> MDTNQKLSIAVFALGCFWGPDAQFGSIKGVVSTRVGYAGGTTNNPSYYNLGDHSESIEIQYDANVITYGELLNIFWNLHNPVYETTNRQYMSRIFYLDDGQKSEALEMKRQIEAANGEKIYTEIVPLENFYLAEGYHQKYYLQNTTKLYQTLKAIYGGFGNLVRSTLAARMNGYIAGNLSIASLKEEMDLVELPEDQYEKVLSIVEEI;>MAKEVIVYTSNTCPHSFTVKEF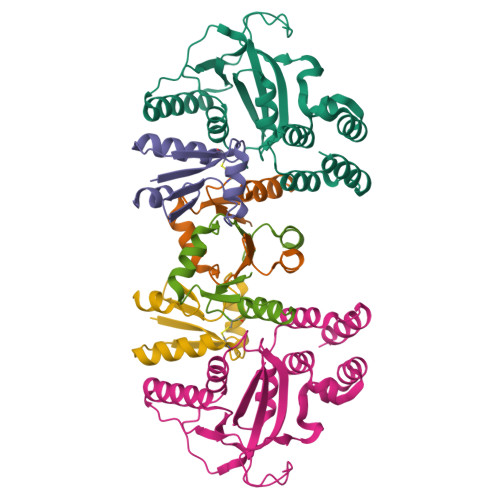LSENNVEFTEKNIQTDAAARKELMKKGIMAVPVIQIDEEVVVGFDRDKIEELLGLEHHHHHH[2x]>MSMSQFFIRRPVFAWVIAIFIIIFGLLSIPKLPIARFPSVAPPQVNISATYPGATAKTINDSVVTLIERELSGVKNLLYYSATTDTSGTAEITATFKPGTDVEMAQVDVQNKIKAVEARLPQVVRQQGLQVEASSSGFLMLVGINSPNNQYSEVDLSDYLVRNVVEELKRVEGVGKVQSFGAEKAMRIWVDPNKLVSYGLSISDVNNAIRENNVEIAPGRLGDLPAEKGQLITIPLSAQGQLSSL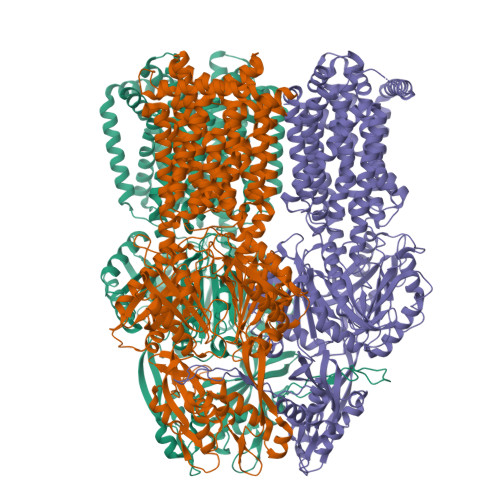EQFKNISLKSKTNGSVIKLSDVANVEIGSQAYNFAILENGKPATAAAIQLSPGANAVKTAEGVRAKIEELKLNLPEGMEFSIPYDTAPFVKISIEKVIHTLLEAMVLVFIVMYLFLHNVRYTLIPAIVAPIALLGTFTVMLLAGFSINVLTMFGMVLAIGIIVDDAIVVVENVERIMATEGLSPKDATSKAMKEITSPIIGITLVLAAVFLPMAFASGSVGVIYKQFTLTMSVSILFSALLALILTPALCATILKPIDGHHQKKGFFAWFDRSFDKVTKKYELMLLKIIKHTVPMMVIFLVITGITFAGMKYWPTAFMPEEDQGWFMTSFQLPSDATAERTRNVVNQFENNLKDNPDVKSNTAILGWGFSGAGQNVAVAFTTLKDFKERTSSASKMTSDVNSSMANSTEGETMAVLPPAIDELGTFSGFSLRLQDRANLGMPALLAAQDELMAMAAKNKKFYMVWNEGLPQGDNISLKIDREKLSALGVKFSDVSDIISTSMGSMYINDFPNQGRMQQVIVQVEAKSRMQLKDILNLKVMGSSGQLVSLSEVVTPQWNKAPQQYNRYNGRPSLSIAGIPNFDTSSGEAMREMEQLIAKLPKGIGYEWTGISLQEKQSESQMAFLLGLSMLVVFLVLAALYESWAIPLSVMLVVPLGIFGAIIAIMSRGLMNDVFFKIGLITIIGLSAKNAILIVEFAKMLKEEGMSLIEATVAAAKLRLRPILMTSLAFTCGVIPLVIATGASSETQHALGTGVFGGMISATILAIFFVPVFFIFILGAVEKLFSSKKKISSALEVLFQGPHHHHHHHHHH[3x]> NGIVPDAGHQGPDVSAVNGGTQVINIVTPNNEGISHNQYQDFNVGKPGAVFNNALEAGQSQLAGHLNANSNLNGQAASLILNEVVSRNPS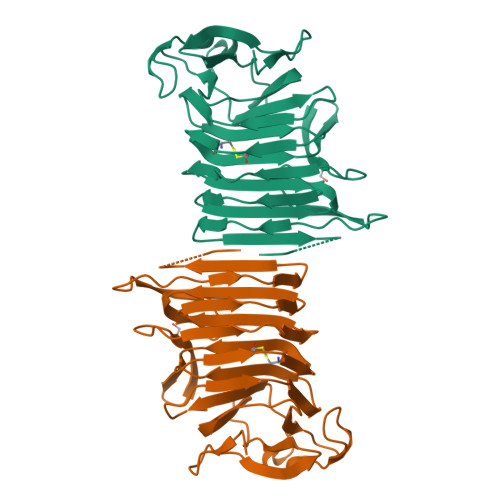FLLGQAEVFGIAAEYVLSNPNGITCDGCGFINTSRSSLVVGNPLFENGQLKGYSTLNNTNLLSLGKNGLNTTGLLDLIAPRIDSRGKITAAEISAFTGQNTFSQHFDILSSQKPVSALDSYFFGSMQSGRIRIINTAEGSGVKLAGHHHHHH> MPKALRFLGWPVLVGVLLALLIIQHNPELVGLPRQEVHVEQAPLLSRLQEGPPSYANAVSRAAPAVANLYTTKMVSKPSHPLFDDPMFRRFFGDNLPQQKRMESSLGSAVIMSAEGYLLTNNHVTAGADQIIVALRDGRETIAQLVGSDPETDLAVLKIDLKNLPAMTLGRSDGIRTGDVCLAIGNPFGVGQTVTMGIISATGRNQLGLNTYEDFIQTDAAINPGNSGGALVDAAGNLIGINTAIFSKSGGSQGIGFA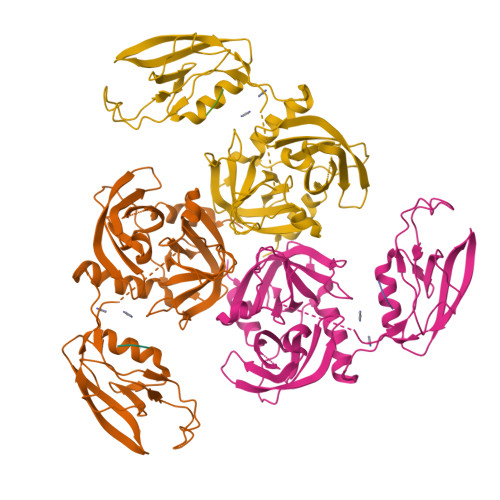IPTKLALEVMQSIIEHGQVIRGWLGVEVKALTPELAESLGLGETAGIVVAGVYRDGPAARGGLLPGDVILTIDKQEASDGRRSMNQVARTRPGQKISIVVLRNGQKVNLTAEVGLRPPPAPAPQQKQDGGE;> WVF>[4x]KVEDPKDFPSELL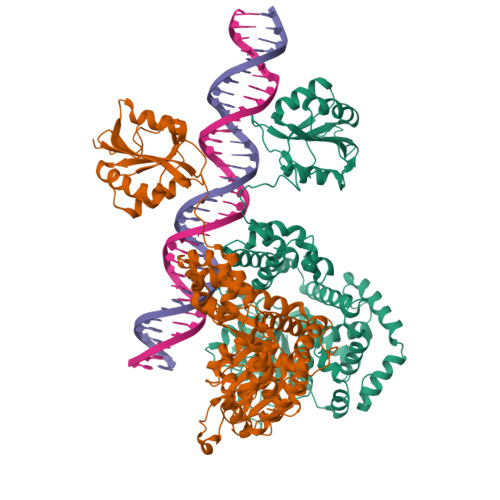SFLSHAVFSNRTLACFAIYTTKEKAALLYKKIMEKYSVTFISRHNSYNHNILFFLTPHRHRVSAINNYAQKLCTFSFLICKGVNKEYLMYSALTRDPFSVIEESLPGGLKEHDFNPEEAEETKQVSWKLVTEYAMETKCDDVLLLLGMYLEFQYSFEMCLKCIKKEQPSHYKYHEKHYANAAIFADSKNQKTICQQAVDTVLAKKRVDSLQLTREQMLTNRFNDLLDRMDIMFGSTGSADIEEWMAGVAWLHCLLPKMDSVVYDFLKCMVYNIPKKRYWLFKGPIDSGKTTLAAALLELCGGKALNVNLPLDRLNFELGVAIDQFLVVFEDVKGTGGESRDLPSGQGINNLDNLRDYLDGSVKVNLEKKHLNKRTQIFPPGIVTMNEYSVPKTLQARFVKQIDFRPKDYLKHCLERSEFLLEKRIIQSGIALLLMLIWYRPVAEFAQSIQSRIVEWKERLDKEFSLSVYQKMKFNVAMGIGVLD>HMGAPATVTEQGEDITSKKDRGVLKIVKRVGNGEETPMIGDKVYVHYKGKLS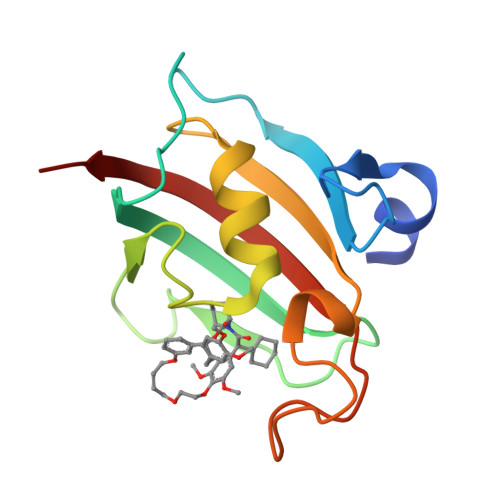NGKKFDSSHDRNEPFVFSLGKGQVIKAWDIGVATMKKGEIAHLLIKPEYAYGSAGSLPKIPSNATLFFEIELLDFKGE[2x]>[2x]GWIKGVLVRCMLNIWGVMLFIRLSWIVGQAGIGLSVLVIMMATVVTTITGLSTSAIATNGFVRGGGAYYLISRSLGPEFGGAIGLIFAFANAVAVAMYVVGFAETVVELLKEHSILMIDEINDIRIIGAITVVILLGISVAGMEWEAKAQIVLLVILLLAIGDFVIGTFIPLESKKPKGFFGYKSEIFNENFGPDFREEETFFSVFAIFFPAATGILAGANISGDLADPQSAIPKGTLLAILITTLVYVGIAVSVGSCVVRDATGNVNDTIVTELTNCTSAACKLNFDFSSCESS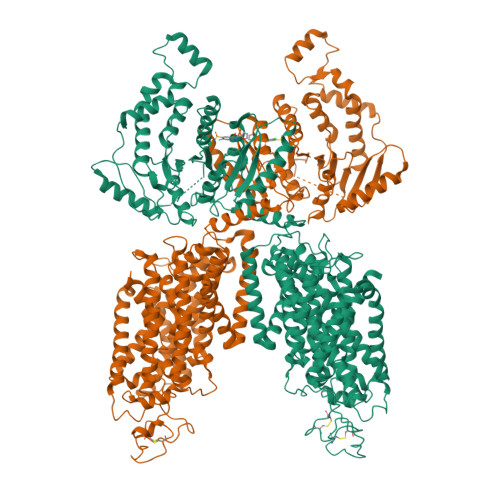PCSYGLMNNFQVMSMVSGFTPLISAGIFSATLSSALASLVSAPKIFQALCKDNIYPAFQMFAKGYGKNNEPLRGYILTFLIALGFILIAELNVIAPIISNFFLASYALINFSVFHASLAKSPGWRPAFKYYNMWISLLGAILCCIVMFVINWWAALLTYVIVLGLYIYVTYKKPDVNWGSSTQALTYLNALQHSIRLSGVEDHVKNFRPQCLVMTGAPNSRPALLHLVHDFTKNVGLMICGHVHMGPRRQAMKEMSIDQAKYQRWLIKNKMKAFYAPVHADDLREGAQYLMQAAGLGRMKPNTLVLGFKKDWLQADMRDVDMYINLFHDAFDIQYGVVVIRLKEGLXXXXXXXXXXXXXXXXXXXXXXXXXXXXXXXXXXXXXXXXXXXXXXXXXXXXXXXXXXXXXXXXXXXXXXXXXXXXXXXXXXXXXXXXXXXKQGKNTIDVWWLFDDGGLTLLIPYLLTTKKKWKDCKIRVFIGGKINRIDHDRRAMATLLSKFRIDFSDIMVLGDINTKPKKENIIAFEEIIEPYRLHEDDKEQDIADKMKEDEPWRITDNELELYKTKTYRQIRLNELLKEHSSTANIIVMSLPVARKGAVSSALYMAWLEALSKDLPPILLVRGNHQSVLTF>MES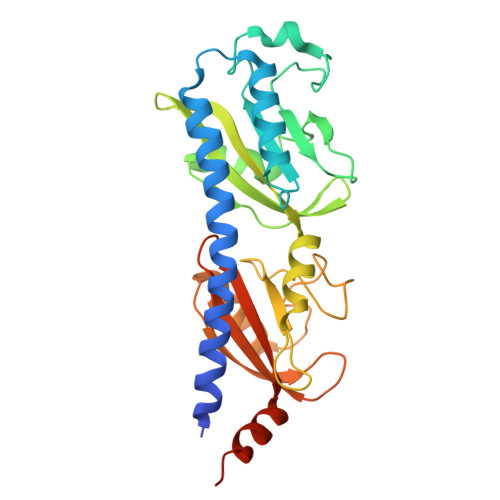TVTTQEEKLAYQQSVEMASNYANQFDADMKANLAIARTISTTMESYETADRDEALLILENLLRDNPHLLGTYVAFEPDAFDGKDAEYTNSPAHDGTGRFVPYWNKMNGTASVAPLLHYDSSDYYQLPKATEKDVLTEPYFYEGVFMVSYVSPIMKEGEFAGIGGVDVSLEYVDEVVSKVRTFDTGYAFMVSNSGVILSHPTHKDWIGKKDLYDFGGEELEKASRDIKNGIGGHLETADPTTGKTVILFYEPVETGDFAFVLVVPKEEMLAGVADLRERLLEHHHHHH[10x]>[2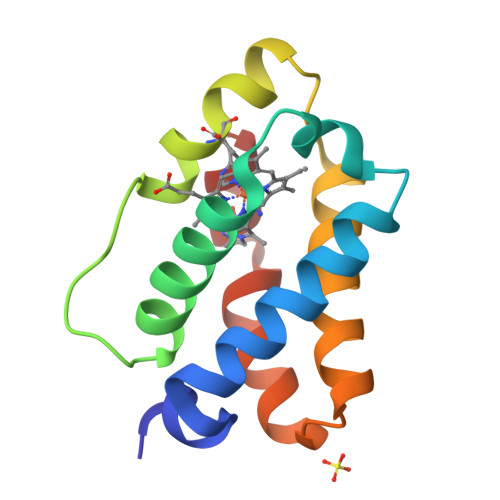x]ASLYEKLGGAAAVDLAVEKFYGKVLADERVNRFFVNTDMAKQKQHQKDFMTYAFGGTDRFPGRSMRAAHQDLVENAGLTDVHFDAIAENLVLTLQELNVSQDLIDEVVTIVGSVQHRNDVLNR>[6x]MHHHHHHMANCERTFIAIKPDGV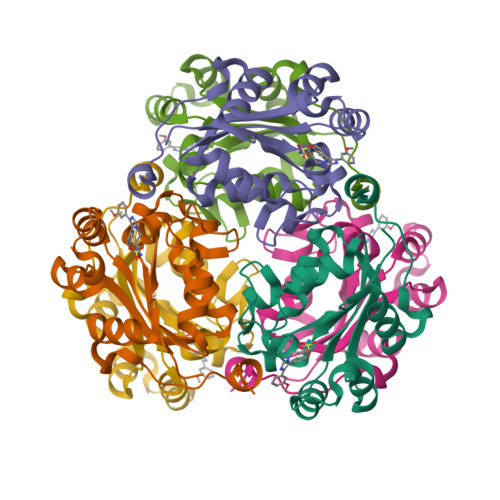QRGLVGEIIKRFEQKGFRLVGLKFMQASEDLLKEHYVDLKDRPFFAGLVKYMHSGPVVAMVWEGLNVVKTGRVMLGETNPADSKPGTIRGDFCIQVGRNIIHGSDSVESAEKEIGLWFHPEELVDYTSCAQNWIYE> GPLGSPPKRLTREAMRNYLKERGDQTVLILHAKVAQKSYGNEKRFFCPPPCVYLMGSGWKKKKEQMERDGCSEQESQPCAFIGIGNSDQEMQQLNLEGKNYCTAKTLYISDSDKRKHFMLSVKMFYGNSDDIGVFLSKRIKVISKPSKKKQSLKNADLCIASGTKVALFNRLRSQTVSTRYLHVEGGNFHASSQQWGAFYIHLLDDDESEGEEFTVRDGYIHYGQTVKLVCSVTGMALPRLIIRKVDKQTALLDADDPVSQLHKCAFYLKDTERMYLC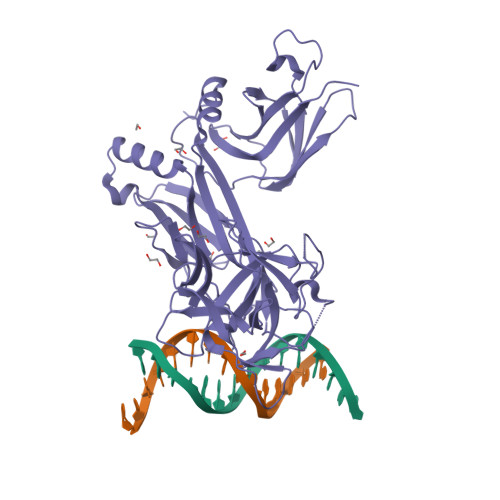LSQERIIQFQATPCPKEQNKEMINDGASWTIISTDKAEYTFYEGMGPVLAPVTPVPVVESLQLNGGGDVAMLELTGQNFTPNLRVWFGDVEAETMYRCGESMLCVVPDISAFREGWRWVRQPVQVPVTLVRNDGVIYSTSLTFTYTPEP>DGGEYLRPEDLKELGDDSLPSSQFLDGMNYLRYSLEGGRSLVPRGSGSRNGITPLHVASKRGNTNMVKLLLDRGGQIDAKTRDGLTPLHCAARSGHDQVVELLLERGA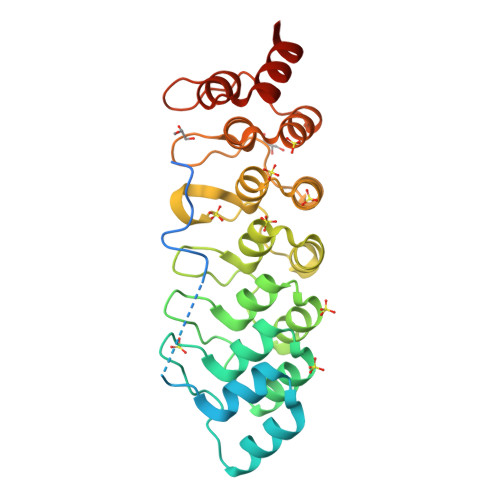PLLARTKNGLSPLHMAAQGDHVECVKHLLQHKAPVDDVTLDYLTALHVAAHCGHYRVTKLLLDKRANPNARALNGFTPLHIACKKNRIKVMELLVKYGASIQAITESGLTPIHVAAFMGHLNIVLLLLQNGASPDVTNIRGETALHMAARAGQVEVVRCLKVVTEEVTT[2x]>MKLPVREFDAVVIGAGGAGMRAALQISQSGQTCALLSKVFPTRSHTVSAQGGITVALGNTHEDNWEWHMYDTVKGSDYIGDQDAIEYMCKTGPEAILELEHMGLPFSRLDDGRIYQRPFGGQSKNFGGEQAARTAAAADRTGHALLHTLYQQNLKNHTTIFSEWYALDLVKNQDGAVVGCTALCIETGEVVYFKARATVLATGGAGRIYQSTTNAHINTGDGVGMAIRAGVPVQDMEMWQFHPTGIAGAGVLVTEGCRGEGGYLLNKHGERFMERYAPNAKDLAGRDVVARSIMIEIREGRGCDGPWGPHAKLKLDHLGKEVLESRLPGILELSRTFAHVDPVKEPIPVIPTCHYMMGGIPTKVTGQALTVNEKGEDVVVPGLFAVGEIACVSVHGANRLGGNSLLDLVVFGRAAGLHLQESIAEQGALRDASESDVEASLDRLNRWNNNRNGEDPVAIRKALQECMQHNFSVFREGDAMAKGLEQLKVIRERLKNARLDDTSSEFNTQRVECLELDNLMETAYATAVSANFRTESRGAHSRFDFPDRDDENWLCHSLYLPESESMTRRSVNMEPKLRPAFPPKIRTY[3x];>MRLEFSIYRYNPDVDDAPRMQDYTLEADEGRDMMLLDALIQLKEKDPSLSFRRSCREGVCGSDGL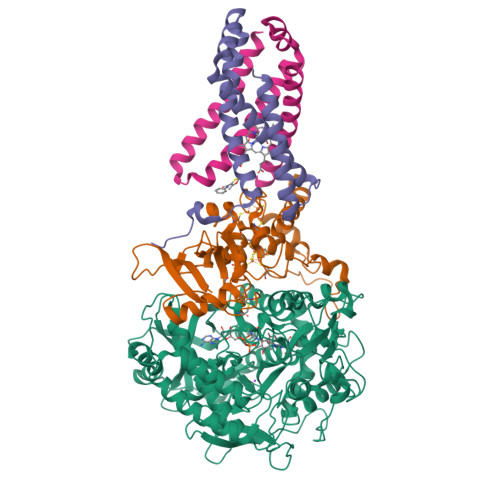NMNGKNGLACITPISALNQPGKKIVIRPLPGLPVIRDLVVDMGQFYAQYEKIKPYLLNNGQNPPAREHLQMPEQREKLDGLYECILCACCSTSCPSFWWNPDKFIGPAGLLAAYRFLIDSRDTETDSRLDGLSDAFSVFRCHSIMNCVSVCPKGLNPTRAIGHIKSMLLQRNA[3x];>MIRNVKKQRPVNLDLQTIRFPITAIASILHRVSGVITFVAVGILLWLLGTSLSSPEGFEQASAIMGSFFVKFIMWGILTALAYHVVVGIRHMMMDFGYLEETFEAGKRSAKISFVITVVLSLLAGVLVW[3x];>[3x]MVSNASALGRNGVHDFILVRATAIVLTLYIIYMVGFFATSGELTYEVWIGFFASAFTKVFTLLALFSILIMAWIGMWQVLTDYVKPLALRLMLQLVIVVALVVYVIYGFVVVWGV> GSHMASMNSEILNNIILNLRYKDNNLIDLSGYGAKVEVYDGVELNDKNQFKLTSSANSKIRVTQNQNIIFNSVFLDFSVSFWIRIPKYKNDGIQNYIHN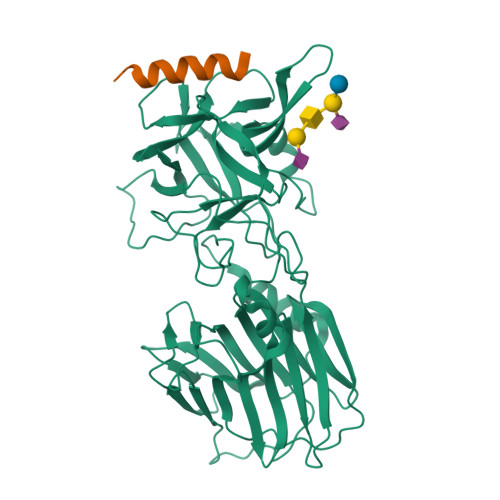EYTIINCMKNNSGWKISIRGNRIIWTLIDINGKTKSVFFEYNIREDISEYINRWFFVTITNNLNNAKIYINGKLESNTDIKDIREVIANGEIIFKLDGDIDRTQFIWMKYFSIFNTELSQSNIEERYKIQSYSEYLKDFWGNPLMYNKEYYMFNAGNKNSYIKLKKDSPVGEILTRSKYNQNSKYINYRDLYIGEKFIIRRKSNSQSINDDIVRKEDYIYLDFFNLNQEWRVYTYKYFKKEEEKLFLAPISDSDEFYNTIQIKEYDEQPTYSCQLLFKKDEESTDEIGLIGIHRFYESGWWFEEYKDYFCISKWYLKEVKRKPYNLKLGCNWQFIPKDEGWTE;> GEGKEDAFSKLKEKFMNELHK>[2x]MRTGNLPANMKKNRVLQIIPYEFNRVIIPVKRGEENTDYVNASFIDGYRQKDSYIASQGPLLHTIEDFWRMIWEWKSCSIVMLTELEERGQEKCAQYWPSDGLVSYGDITVELKKEEECES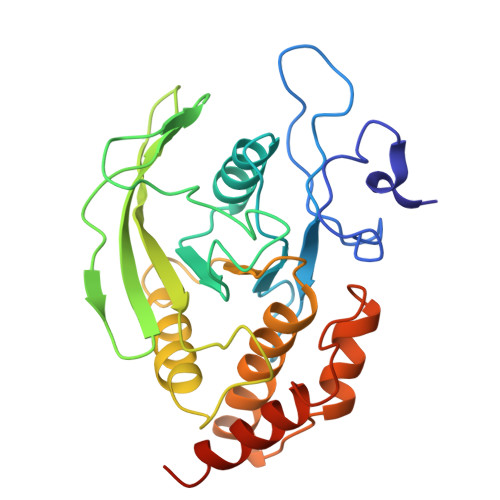YTVRDLLVTNTRENKSRQIRQFHFHGWPEVGIPSDGKGMINIIAAVQKQQQQSGNHPITVHCSAGAGRTGTFCALSTVLERVKAEGILDVFQTVKSLRLQRPHMVQTLEQYEFCYKVVQEYIDAFSDYANFK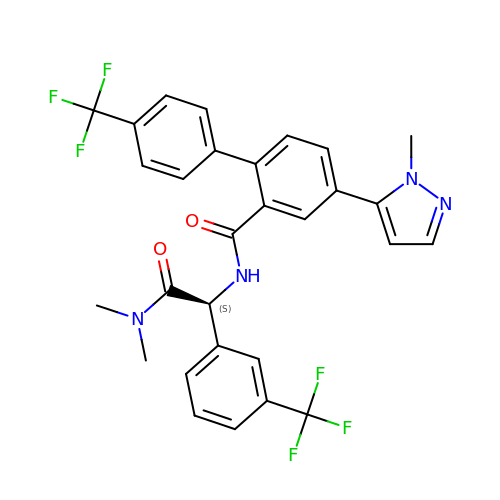(4M)-N-{(1S)-2-(dimethylamino)-2-oxo-1-[3-(trifluoromethyl)phenyl]ethyl}-4-(1-methyl-1H-pyrazol-5-yl)-4'-(trifluoromethyl)[1,1'-biphenyl]-2-carboxamide | C29 H24 F6 N4 O2 | KNKLXKBJJSPVFJ-VWLOTQADSA-N3,4-Dihydroxyphenylalanine (DOPA) decarboxylase (DDC) is a pyridoxal-5′-phophate (PLP)-dependent enzyme which physiologically catalyzes the decarboxylation of 3,4-dihydroxyphenylalanine to dopamine, and 5-hydroxytryptophan (5-HTP) to 5-hydroxytryptamine (serotonin). Because the enzyme catalyzes the decarboxylation of other aromatic L-amino acids as well, it is commonly named aromatic L-amino acid decarboxylase. In insects DDC occupies a special position because dopamine is a key precursor in insect cuticle formation, eggshell hardening and is involved in immune responses. In this study, we determined the crystal structure of the typical Drosophila DDC (drDDC).

The structure of drDDC was determined by molecular replacement and refined to 1.75 Å resolution with excellent statistics. There are two protein molecules in an asymmetric unit, which forms a biological homodimer. The fragment of V322 to P348 of both subunits in the structure was highly disordered; therefore, they were not included in the final drDDC model. Each of the two monomers is composed of three distinct domains. The large domain (Residues 86–380) contains a seven-stranded beta sheet, and the small domain comprises the C-terminal part of the chain (residues 380–475), which folds into a 4-stranded beta sheet covered with helices on one side. Based on the above features of the structure, drDDC is a fold-type I PLP-dependent enzyme. The active site of drDDC is located near the monomer-monomer interface but is composed mainly of residues from one monomer. The cofactor PLP binds to K302 through a Schiff base linkage to form an internal aldimine, lysine-pyridoxal-5-phosphate (LLP). The carboxyl group of D270 and the protonated pyridine nitrogen of PLP form a pair of salt bridges, which is structurally and functionally conserved within fold-type I of the PLP-dependent enzyme family. The PLP pyridine ring is stacked between residues A272 on one side and H192 on the other side. Upon superposing the native drDDC structure onto the pig DDC structure, we identified a flexible loop in drDDC structure, which did not superpose well.

>[2x]MEAPEFKDFAKTMVDFIAEYLENIRERRVLPEVKPGYLKPLIPDAAPEKPEKWQDVMQDIERVIMPGVTHWHSPKFHAYFPTANSYPAIVADMLSGAIACIGFTWIASPACTELEVVMMDWLGKMLELPAEFLACSGGKGGGVIQGTASESTLVALLGAKAKKLKEVKELHPEWDEHTILGKLVGYCSDQAHSSVERAGLLGGVKLRSVQSENHRMRGAALEKAIEQDVAEGLIPFYAVVTLGTTNSCAFDYLDECGPVGNKHNLWIHVDAAYAGSAFICPEYRHLMKGIESADSFNFNPHKWMLVNFDCSAMWLKDPSWVVNAFNVDPLYLKHDMQGSAPDYRHWQIPLGRRFRALKLWFVLRLYGVENLQAHIRRHCNFAKQFGDLCVADSRFELAAEINMGLVCFRLKGSNERNEALLKRINGRGHIHLVPAKIKDVYFLRMAICSRFTQSEDMEYSWKEVSAAADEMEQEQ> VPKLTASVTDGAVGVTVDAPVSVTAADGVLAAVTMVNDNGRPVAGRLSPDGLRWSTTEQLGYNRRYTLNATALGLGGAATRQLTFQTSSPAHLTMPYVMPGDGEVVGVGEPVAIRFDENIADRGAAEKAIKITTNPPVEGAFYWLNNREVRWRPEHFWKPGTAVDVAVNTYGVDLGEGMFGEDNVQTHFTIGDEVIATADDNTKILTVRVNGEVVKSMPTSMGKDSTPTANGIYIVGSRYKHIIMDSSTYGVPVNSPNGYRTDVDWATQISYSGVFVHSAPWSVGAQGHTNTS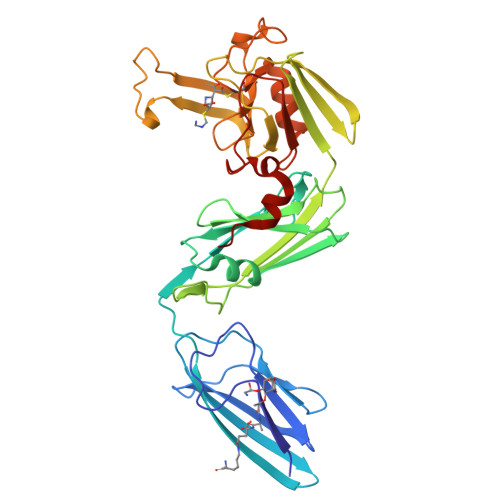HGCLNVSPSNAQWFYDHVKRGDIVEVVNTVGGTLPGIDGLGDWNIPWDQWRAGNAK>[4x]MQIRKKTIVCMLLFILFVGNAVAQQNITNVYGRDIRSLNGKWNAIIDLYDQGRGMKVYRNQSPKGNTDFYEYSFQGGLRLNVPGDWNSQTPELKYYEGTVWYARHFDAKRLTHKRQFLYFG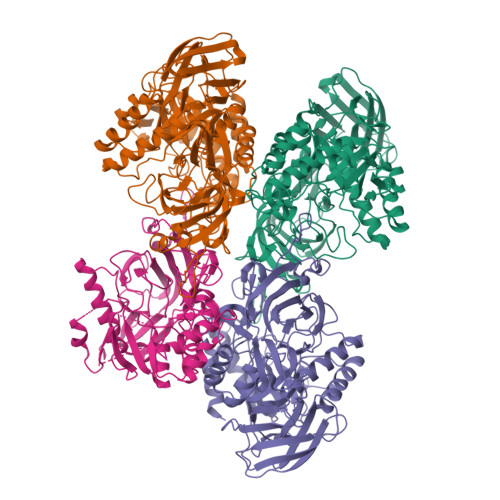AVSYRCRVYLNGAEIGSHEGGFTPFQIEVTDLLNEGENFIAIEVNNRRTKDAIPAMSFDWWNYGGITRDVLLVTTPQTYLEDYFIQLDKESPNRMIAKVALSDKKAGEKITVSIPELKTSIDMLTDAEGKAETVFNIKKLERWSSENPKLYEVIVSSANDRVEEQIGFRNITVKGTDIYLNGKPTFMCSISFHEEIPQRMGRAFSEADAAMLLNEAKALGVNMIRLAHYPQNEYTVRLAEKMGFILWQEIPVWQGIDFTNNNTRKKAQRMLSEMIKRDQNRCAVGYWGIANETQPSKARNEFLTSLLETGKQLDTTRLYVAAFDLVRFNREKKRFVMEDSFTSQLDVVAVNKYMGWYHPWPIEPENAVWEVIPDKPLIISEFGGEALYGQSGDENVASSWSEEYQARLYRDNIRMFDNIPNLRGVSPWILFDFRSPFRFHPTNQDGWNRKGLVSDQGIRKKAWYLMREYYKTKFGE>MGKSLSHLPLHSSKEDAYDGVTSENMRNGLVNSEVHNEDGRNGDVSQFPYVEFTGRDSVTCPTCQGTGRIPRGQENQLVALIPYSDQRLRPRRTKLYVMASVFVCLLLSGLAVFFLFPRSIDVKYIGVKSAYVSYDVQKRTIYLNITNTLNITNNNYYSVEVENITAQVQFSKTVIGKARLNNITIIGPLDMKQIDYTVPTVIAEEMSY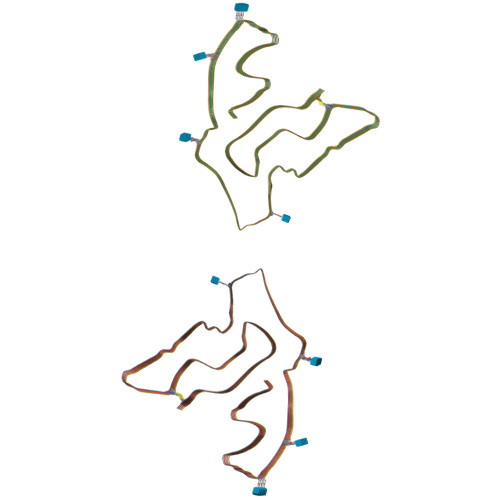MYDFCTLISIKVHNIVLMMQVTVTTTYFGHSEQISQERYQYVDCGRNTTYQLGQSEYLNVLQPQQ[10x]> AAPTATVTPSSGLSDGTVVKVAGAGLQAGTAYWVAQWARVDTGVWAYNPADNSSVTADANGSASTSLTVRRSFEGFLFDGTRWGTVDCTTAACQVGLSDAAGNGPEG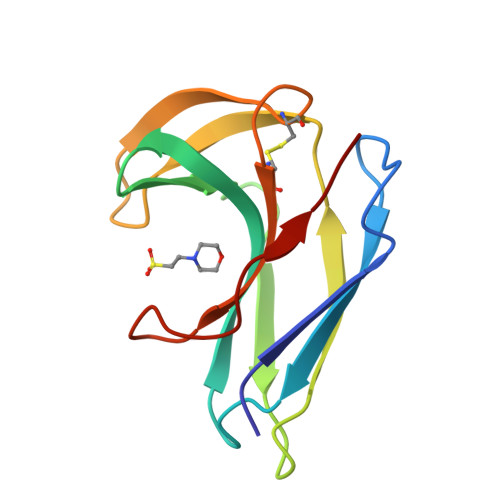VAISF> MSQSNRELVVDFLSYKLSQKGYSWSQFSDVEENRTEAPEGTESEMETPSAINGNPSWHLADSPAVNGATGHSSSLDAREVIPMAAVKQALREAGDEFELRYRRAFSDLTSQLHITPGTAYQSFEQVVNELFRDGVNAGRIVAFFSFGGALCVESVDKEMQVLVSRIAAWMA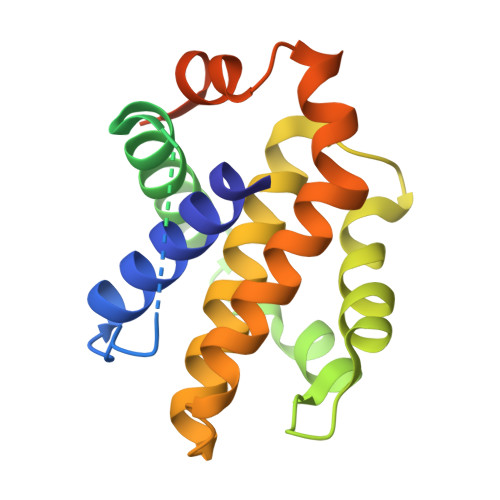TYLNDHLEPWIQENGGWDTFVELYGNNAAAESRKGQERFNLEHHHHHH>AAMTLASQIATQLLD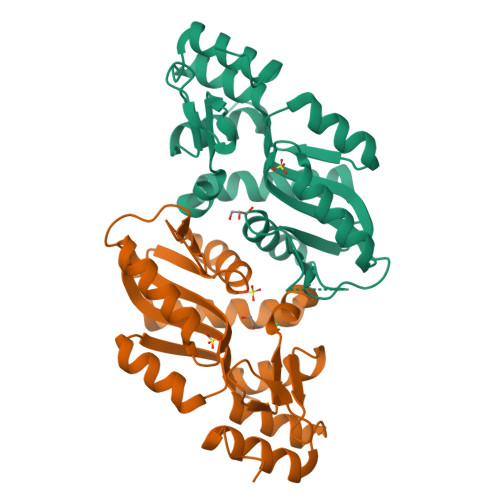IKAVYLKPEDPFTWASGIKSPIYTDNRVTLSYPKTRDLIENGFVETIKAHFPEVEVIAGTATAGIPHGAIIADKMTLPFAYIRSKPKDHGAGNQIEGRVLKGQKMVIIEDLISTGGSVLDAAAAASREGADVLGVVAIFTYELPKASQNFKEAGIKLITLSNYTELIAVAKLQGYITNDGLHLLKKFKEDQVNWQQ[2x]7-{[3-({[(pyridin-2-yl)methyl]amino}methyl)phenoxy]methyl}quinolin-2-amine | C23 H22 N4 O | 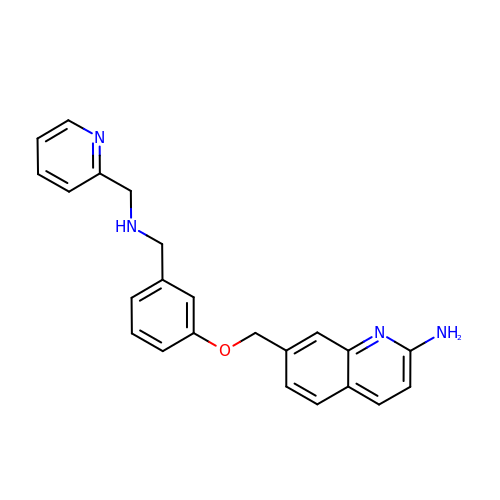MZJVFMHLRQGSTA-UHFFFAOYSA-N(2S)-2-amino-4-(2-aminophenyl)-4-oxobutanoic acid | C10 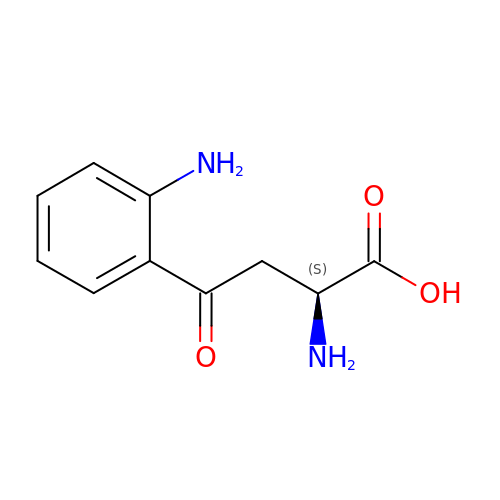H12 N2 O3 | YGPSJZOEDVAXAB-QMMMGPOBSA-N>MEFTTGLMSLDTALNEMLSRVTPLTAQETLPLVQCFGRILASDVVSPLDVPGFDNSAMDGYAVRLADIASGQPLPVAGKSFAGQPYHGEWPAGTCIRIMTGAPVPEGC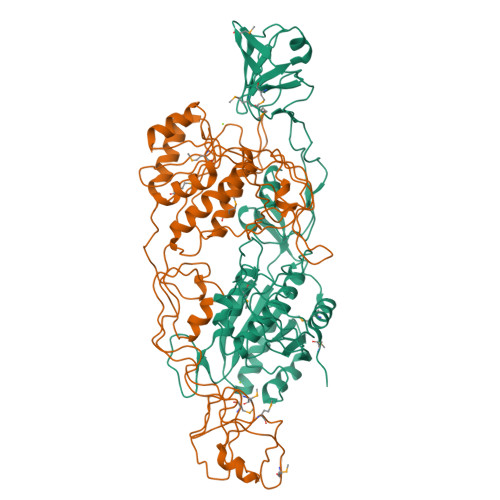EAVVMQEQTEQMDNGVRFTAEVRSGQNIRRRGEDISAGAVVFPAGTRLTTAELPVIASLGIAEVPVIRKVRVALFSTGDELQLPGQPLGDGQIYDTNRLAVHLMLEQLGCEVINLGIIRDDPHALRAAFIEADSQADVVISSGGVSVGEADYTKTILEELGEIAFWKLAIKPGKPFAFGKLSNSWFCGLPGNPVSATLTFYQLVQPLLAKLSGNTASGLPARQRVRTASRLKKTPGRLDFQRGVLQRNADGELEVTTTGHQGSHIFSSFSLGNCFIVLERDRGNVEVGEWVEVEPFNALFGGL[2x]> MTAAPASPQQIRDRLLQAIDPQSNIRNMVAVLEVISSLEKYPITKEALEETRLGKLINDVRKKTKNEELAKRAKKLLRSWQKLIEPAHQHEAALRGLAGATGSANGGAHNCRPEVGAAGPPRSIHDLKSRNDLQRLPGQRLDRLGSRKRRGDQRDLGHPGPPPKVSKASHDPLVPNSSPLPTNGISGSPESFASSLDGSGHAGPEGSRLERDENDKHSGKIPVNAVRPHTSSPGLGKPPGPCLQPKASVLQQLDRVDETPGPPHPKGPPRCSFSPRNSRHEGSFARQQSLYAPKGSVPSPSPRPQALDATQVPSPLPLAQPSTPPVRRLELLPSAESPVCWLEQPESHQRLAGPGCKAGLSPAEPLLSRAGFSPDSSKADSDAASSGGSDSKKKKRYRPRDYTVNLDGQVAEAGVKPVRLKERKLTFDPMTRQIKPLTQKEPVRADSPVHMEQQSRTELDKQEAKASLQSPFEQTNWKELSRNEIIQSYLSRQSSLLSSSGAQTPGAHHFMSEYLKQEESTRQGARQLHVLVPQSPPTDLPGLTREVTQDDLDRIQASQWP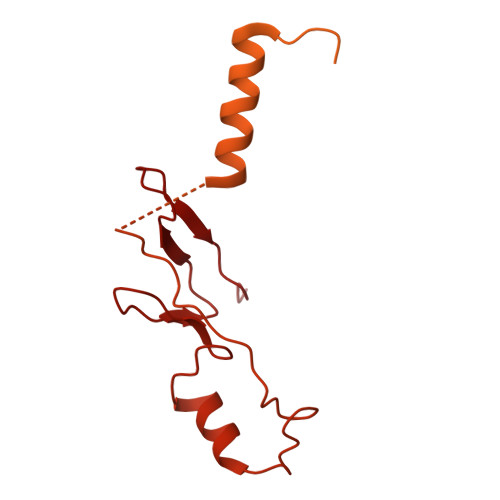GVNGCQDTQGNWYDWTQCISLDPHGDDGRLNILPYVCLD>[2x]VTAVV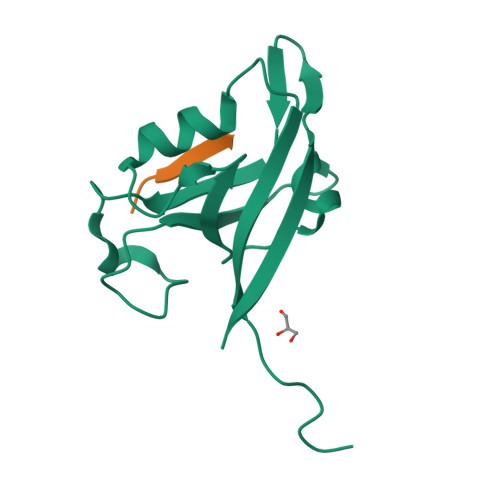QRVEIHKLRQGENLILGFSIGGGIDQDPSQNPFSEDKTDKGIYVTRVSEGGPAEIAGLQIGDKIMQVNGWDMTMVTHDQARKRLTKRSEEVVRLLVTRQSLQKAVQQ;>YPTSII[2x]>MAHHHHHHSAALEVLFQGPGSMSLKVNILGHEFSNPFMNAAGVLCTTEEDLRRMTESESGSLIGKSCTLAPRTGNPEPRYFGLPLGSINSMGLPNLGVDFYLSYAAQTHDYSRKPLFLSMSGLSVEESVEMVKKLVPITKEKGTILELNLSCPNVPGKPQVGYDFDTTRTYLQKVSEAYGLPFGVKMPPYFDIAHFDMAAAVLNDFPLVKFITCVNSIGNGLVIDPANETVVIKPKQGFGGLGGKYVLPTALANVNAFFRRCP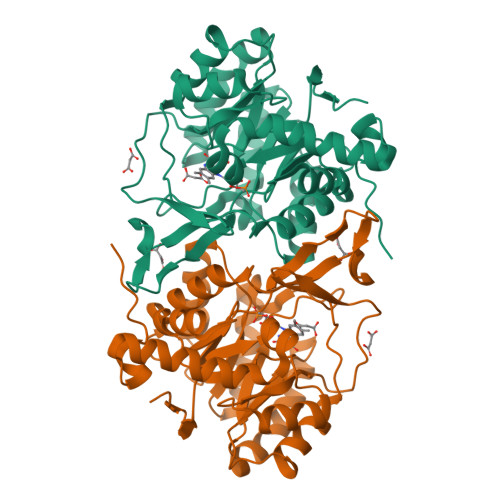DKLVFGCGGVYSGEEAFLHILAGASMVQVGTALHDEGPIIFARLNKELQEIMTNKGYKTLDEFRGRVKTMD[4x]>[2x]VDSESLSEGLVEHVNEVQQQLMKTRKKRPIPQGWATADDVAALQQVAYTDLNVTQASSLDLENECAAVGGLDGKLDIYSVVANKVER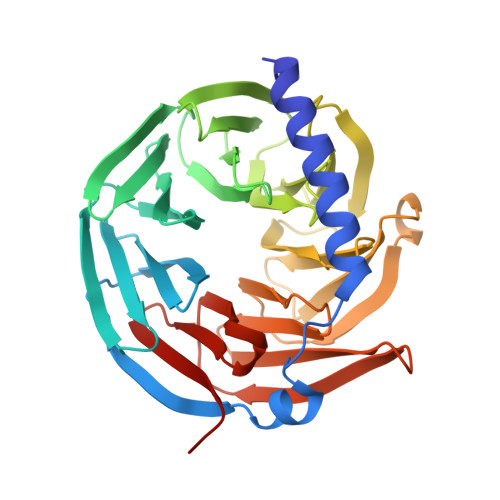TLDIGEPVTATEWTGTKVVIGTAKGWVKVYDAGRESATFQTHAGPVTGLAVHPGGRILASVGVDKSFVFYDLETGERVARGYADAALTTCAFHPDGNLFAAGTQTGHILVFHTTTLEQAESFPLGTPIQALAFSENGFWFAATGKGTSSVTIFDLRKSGAAAAVKELQTGEVLSISWDYTGQYLATGGGTGVTVQMYTKATKSWSEPVRLGMPVVGVKWGGEAKRLVVVSREGVVSVLGKKE>MEEVVLITVPSEEVARTIAKALVEERLAACVNIVPGLTSIYRWQGEVVEDQELLLLVKTTTHAFPKLKE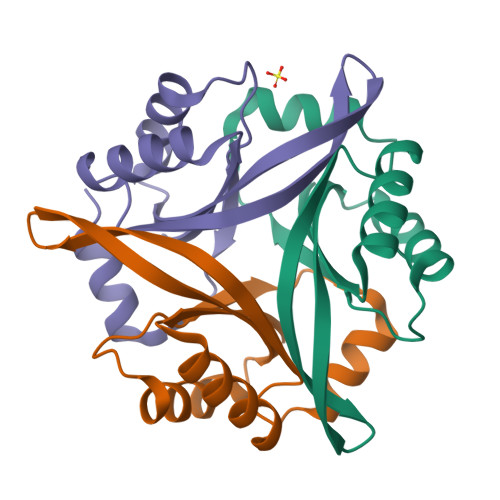RVKALHPYTVPEIVALPIAEGNREYLDWLRENTG[3x]> MNLEVLCGRINVENGLSLGEPGLYDQIYDRPGLPD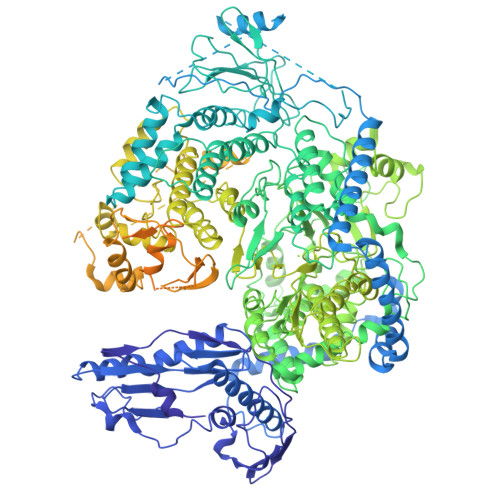LDVTVDATGVTVDIGAVPDSASQLGSSINAGLITIQLSEAYKINHDFTFSGLSKTTDRRLSEVFPITHDGSDGMTPDVIHTRLDGTIVVVEFSTTRSHNIGGLEAAYRTKIEKYRDPISRRVDIMENPRVFFGVIVVSSGGVLSNMPLTQDEAEELMYRFCIANEIYTKARSMDADIELQKSEEELEAISRALSFFSLFEPNIERVEGTFPNSEIKMLEQFLSTPADVDFITKTLKAKEVEAYADLCDSHYLKPEKTIQERLEINRCEAIDKTQDLLAGLHARSNKQTSLNRGTVKLPPWLPKPSSESIDIKTDSGFGSLMDHGAYGELWAKCLLDVSLGNVEGVVSDPAKELDIAISDDPEKDTPKEAKITYRRFKPALSSSARQEFSLQGVEGKKWKRMAANQKKEKESHETLSPFLDVEDIGDFLTFNNLLTDSRYGDESIQRAVSILLEKASAMQDTELTHALNDSFKRNLSSNVVQWSLWVSCLAQELASALKQHCRAGEFIIKKLKFWPIYVIIKPTKSSSHIFYSLGIRKADVTRRLTGRVFSDTIDAGEWELTEFKSLKTCKLTNLVNLPCTMLNSIAFWREKLGVAPWLVRKPCSELREQVGLTFLISLEDKSKTEEIITLTRYTQMEGFVSPPMLPKPQKMLGKLDGPLRTKLQVYLLRKHLDCMVRIASQPFSLIPREGRVEWGGTFHAISGRSTNLENMVNSWYIGYYKNKEESTELNALGEMYKKIVEMEEDKPSSPEFLGWGDTDSPKKHEFSRSFLRAACSSLEREIAQRHGRQWKQNLEERVLREIGTKNILDLASMKATSNFSKDWELYSEVQTKEYHRSKLLEKMATLIEKGVMWYIDAVGQAWKAVLDDGCMRICLFKKNQHGGLREIYVMDANARLVQFGVETMARCVCELSPHETVANPRLKNSIIENHGLKSARSLGPGSININSSNDAKKWNQGHYTTKLALVLCWFMPAKFHRFIWAAISMFRRKKMMVDLRFLAHLSSKSESRSSDPFREAMTDAFHGNRDVSWMDKGRTYIKTETGMMQGILHFTSSLLHSCVQSFYKSYFVSKLKEGYMGESISGVVDVIEGSDDSAIMISIRPKSDMDEVRSRFFVANLLHSVKFLNPLFGIYSSEKSTVNTVYCVEYNSEFHFHRHLVRPTLRWIAASHQISETEALASRQEDYSNLLTQCLEGGASFSLTYLIQCAQLLHHYMLLGLCLHPLFGTFMGMLISDPDPALGFFLMDNPAFAGGAGFRFNLWRACKTTDLGRKYAYYFNEIQGKTKGDEDYRALDATSGGTLSHSVMVYWGDRKKYQALLNRMGLPEDWVEQIDENPGVLYRRAANKKELLLKLAEKVHSPGVTSSLSKGHVVPRVVAAGVYLLSRHCFRFSSSIHGRGSTQKASLIKLLMMSSISAMKHGGSLNPNQERMLFPQAQEYDRVCTLLEEVEHLTGKFVVRERNIVRSRIDLFQEPVDLRCKAEDLVSEVWFGLKRTKLGPRLLKEEWDKLRASFAWLSTDPSETLRDGPFLSHVQFRNFIAHVDAKSRSVRLLGAPVKKSGGVTTISQVVRMNFFPGFSLEAEKSLDNQERLESISILKHVLFMVLNGPYTEEYKLEMIIEAFSTLVIPQPSEVIRKSRTMTLCLLSNYLSSRGGSILDQIERAQSGTLGGFSKPQKTFVRPGGGVGYKGKGVWTGVMEDTHVQILIDGDGTSNWLEEIRLSSDARLYDVIESIRRLCDDLGINNRVASAYRGHCMVRLSGFKIKPASRTDGCPVRIMERGFRIRELQNPDEVKMRVRGDILNLSVTIQEGRVMNILSYRPRDTDISESAAAYLWSNRDLFSFGKKEPSCSWICLKTLDNWAWSHASVLLANDRKTQGIDNRAMGNIFRDCLEGSLRKQGLMRSKLTEMVEKNVVPLTTQELVDILEEDIDFSDVIAVELSEGSLDIESIFDGAPILWSAEVEEFGEGVVAVSYSSKYYHLTLMDQAAITMCAIMGKEGCRGLLTEKRCMAAIREQVRPFLIFLQIPEDSISWVSDQFCDSRGLDEESTIMWG> MHHHHHHGGGSENLYFQSPGSAAKGSELSERIESFVETLKRGGGPRSSEEMARETLGLLRQIITDHRWSNAGELMELIRREGRRMTAAQPSETTVGNMVRRVLKIIREEYGRLHGRSDESDQQESLHKLLTSGGLNEDFSFHYAQL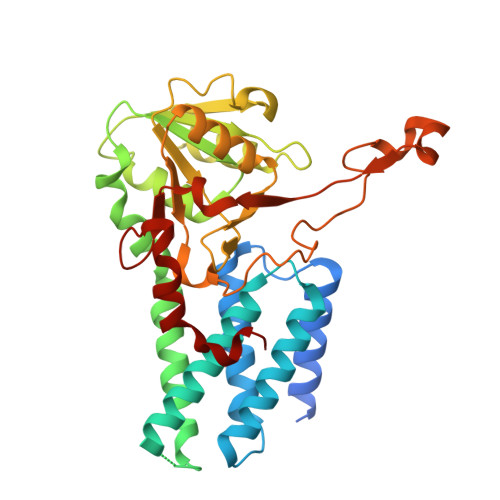QSNIIEAINELLVELEGTMENIAAQALEHIHSNEVIMTIGFSRTVEAFLKEAARKRKFHVIVAECAPFCQGHEMAVNLSKAGIETTVMTDAAIFAVMSRVNKVIIGTKTILANGALRAVTGTHTLALAAKHHSTPLIVCAPMFKLSPQFPNEEDSFHKFVAPEEVLPFTEGDILEKVSVHCPVFDYVPPELITLFISNIGGNAPSYIYRLMSELYHPDDHVL>GMSMPNHPNLTTADAKKILNKFNCLDIAPILKPSEKESVRRALILITKLSDYQILGICADTADEGLLAMKTYSHALGYEVPIDLPVVEGPVYIKLNGKNGLCYLDSYAGHHRGVLVSCQSYYEGGINEMY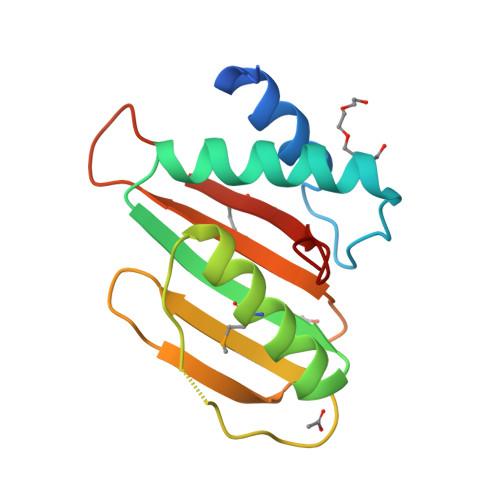GHLPLDLFV[3x]>[8x]GMRKHPQTATKHLFVSGGVASSLGKGLTASSLGQLLTARGLHVTMQKLDPYLNVDPGTMNPFQHGEVFVTEDGAETDLDVGHYERFLDRNLPGSANVTTGQVYSTVIAKERRGEYLGDTVQVIPHITDEIKRRILAMAQPDADGNRPDVVITEIGGTVGDIESQPFLEAARQVRHYLGREDVFFLHVSLVPYLAPSGELKTKPTQHSVAALRSIGITPDALILRCDRDVPEALKNKIALMCDVDIDGVISTPDAPSIYDIPKVLHREELDAFVVRRLNLPFRDVDWTEWDDLLRRVHEPHETVRIALVGKYVELSDAYLSVAEALRAGGFKHRAKVEICWVASDGCETTSGAAAALGDVHGVLIPGGFGIRGIEGKIGAIAYARARGLPVLGLCLGLQCIVIEAARSVGLTNANSAEFDPDTPDPVIATMPDQEEIVAGEADLGGTMRLGSYPAVLEPDSVVAQAYQTTQVSERHRHRYEVNNAYRDKIAESGLRFSGTSPDGHLVEFVEYPPDRHPFVVGTQAHPELKSRPTRPHPLFVAFVGAAIDYKAGELLPVEIPEIPEHTPNGSSHRDGVGQPLPEPASRG

The combined data indicate that 7947882 and 7904688 are prodrugs activated by the EthA monooxygenase, which then target PyrG, a cytidine triphosphate (CTP) synthetase catalyzing the ATP-dependent amination of uridine triphosphate (UTP) to form the essential pyrimidine nucleotide CTP. The crystal structure of PyrG was solved by molecular replacement on a 2.0-Å resolution data set. This structure showed a bidomain enzyme with an N-terminal amidoligase (ALase) domain, also commonly known as the synthetase domain (residues 1–278), connected through an interdomain linker (residues 279–Pro298) to a C-terminal glutamine amidotransferase (GATase) domain (residues 299–552), both domains displaying a Rossmann-like fold. On the other hand, the 34-residue C-terminal extension of M. tuberculosis PyrG, which has no predicted secondary structure or known function, could not be traced due to the lack of supporting electron density, suggesting a high degree of flexibility.

Indeed, another structure of the enzyme in the apo form at lower resolution (3.5 Å), revealed a homodimeric protein, each homodimer representing half of the functional tetramer and showing a dimerization surface of ∼1,350 Å2 per monomer, all in good agreement with previous structural studies (Endrizzi et al., 2004, 2005; Goto et al., 2004; Lauritsen et al., 2011).> MKTSDANETEDHLESLICKVGEKSACSLESNLEGLAGVLEADLPNYKSKILRLLCTVARLLPEKLTIYTTLVGLLNARNYNFGGEFVEAMIRQLKESLKANNYNEAVYLVRFLSDLVNCHVIAAPSMVAMFENFVSVTQEEDVPQVRRDWYVYAFLSSLPWVGKELYEKKDAEMDRIFANTESYLKRRQKTHVPMLQVWTADKPHPQEEYLDCLWAQIQKLKKDRWQERHILRPYLAFDSILCEALQHNLPPFTPPPHTEDSVYPMPRVIFRMFDYTDDPEGPVMPGSHSVERFVIEENLHCIIKSHWKERKTCAAQLVSYPGKNKIPLNYHIVEVIFAELFQLPAPPHIDVMYTTLLIELCKLQPGSLPQVLAQATEMLYMRLDTMNTTCVDRFINWFSHHLSNFQFRWSWEDWSDCLSQDPESPKPKFVREVLEKCMRLSYHQRILDIVPPTFSALCPANPTCIYKYGDESSNSLPGHSVALCLAVAFKSKATNDEIFSILKDVPNPNQDDDDDEGFSFNPLKIEVFVQTLLHLAAKSFSHSFSALAKFHEVFKTLAESDEGKLHVLRVMFEVWRNHPQMIAVLVDKMIRTQIVDCAAVANWIFSSELSRDFTRLFVWEILHSTIRKMNKHVLKIQKELEEAKEKLARQHKRRSDDDDRSSDRKDGVLEEQIERLQEKVESAQSEQKNLFLVIFQRFIMILTEHLVRCETDGTSVLTPWYKNCIERLQQIFLQHHQIIQQYMVTLE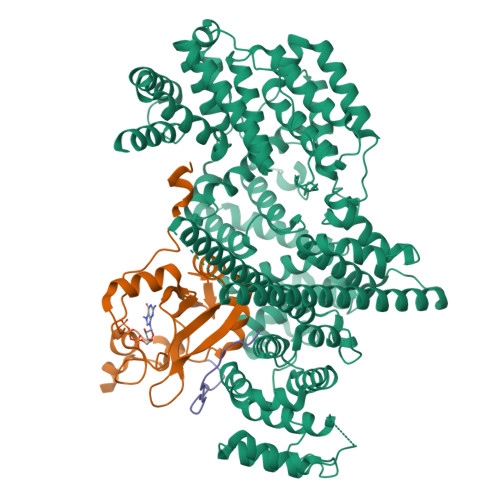NLLFTAELDPHILAVFQQFCALQA;> MSGGLLKALRSDSYVELSQYRDQHFRGDNEEQEKLLKKSCTLYVGNLSFYTTEEQIYELFSKSGDIKKIIMGLDKMKKTACGFCFVEYYSRADAENAMRYINGTRLDDRIIRTDWDAGFKEGRQYGRGRSGGQVRDEYRQDYDAGRGGYGKLAQNQ;> VMKTFKEFLLSLDDSVDETEAVKRYNDYKLDFRRQQMQDFFLAHKDEEWFRSKYHPDEVGKRRQEARGALQNRLRVFLSLMETGWFDNLLLDIDKADAIVKMLDAAVIKMEGGTENDLRILEQEEEEEQAGKPGEPSKKEEGRAGAGLGDGERKTNDKDEKKEDGKQAENDSSNDDKTKKSEGDGDKEEKKEDSEKEAKKSSKKRNRKHSGDDSFDEGSVSESESESESGQAEEEKEEAEEALKEKEKPKEEEWEKPKDAAGLECKPRPLHKTCSLFMRNIAPNISRAEIISLCKRYPGFMRVALSEPQPERRFFRRGWVTFDRSVNIKEICWNLQNIRLRECELSPGVNRDLTRRVRNINGITQHKQIVRNDIKLAAKLIHTLDDRTQLWASEPGTPPLPTSLPSQNPILKNITDYLIEEVSAEEEELLGSSGGAPPEEPPKEGNPAEINVERDEKLIKVLDKLLLYLRIVHSLDYYNTCEYPNEDEMPNRCGIIHVRGPMPPNRISHGEVLEWQKTFEEKLTPLLSVRESLSEEEAQKMGRKDPEQEVEKFVTSNTQELGKDKWLCPLSGKKFKGPEFVRKHIFNKHAEKIEEVKKEVAFFNNFLTDAKRPALPEIKPAQPPGPAQILPPGLTPGLPYPHQTPQGLMPYGQPRPPILGYGAGAVRPAVPTGGPPYPHAPYGAGRGNYDAFRGQGGYPGKPRNRMVRGDPRAIVEYRDLDAPDDVDFF>MELIRFSISIPSKL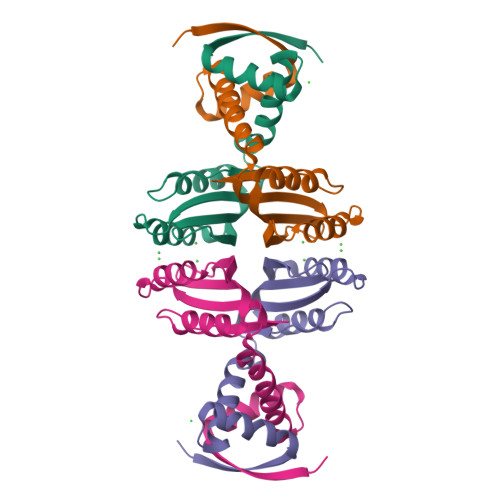LEKFDQIIEEIGYENRSEAIRDLIRDFIIRHEWEVGNEEVAGTITIVYNHDEGDVVKALLDLQHEYLDEIISSLHVHMDEHNCLEVIVVKGEAKKIKMIADKLLSLKGVKHGKLVMTSTGKELV[2x]>[8x]SNRLDGKVAIITGGTLGIGLAIATKFVEEGAKVMITDR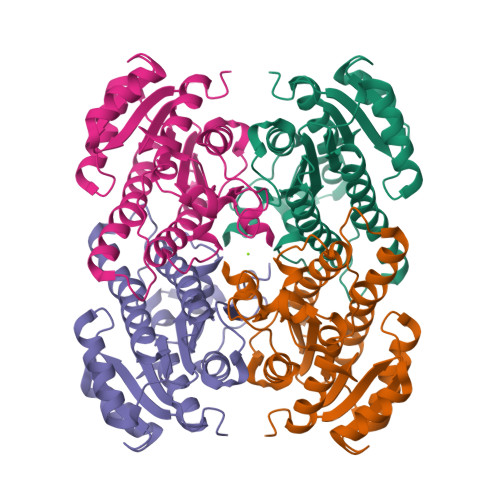HSDVGEKAAKSVGTPDQIQFFQHDSSDEDGWTKLFDATEKAFGPVSTLVNNAGIAVNKSVEETTTAEWRKLLAVNLDGVFFGTRLGIQRMKNKGLGASIINMSSIEGFVGDPSLGAYNASKGAVRIMSKSAALDCALKDYDVRVNTVHPGYIKTPLVDDLPGAEEAMSQRTKTPMGHIGEPNDIAYICVYLASNESKFATGSEFVVDGGYTAQ> DPGCSELIQASSRITTCSTEGVNTKCRLSGTALIRAGSVGAEACLMLKGVKEDQTKFLKIKTVSSELSCREGQSYWTGSFSPKCLSSRRCHLVGECHVNRCLSW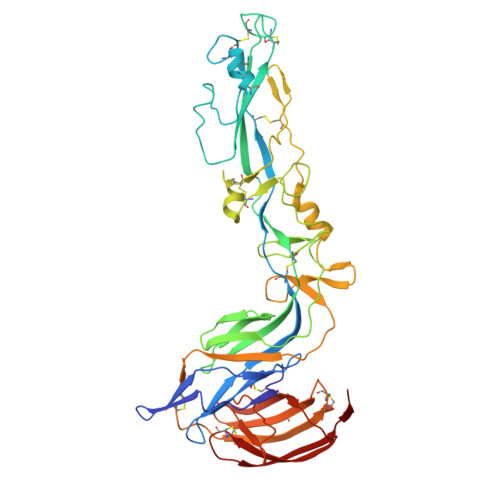RDNETSAEFSFVGESTTMRENKCFEQCGGWGCGCFNVNPSCLFVHTYLQSVRKEALRVFNCIDWVHKLTLEITDFDGSVSTIDLGASSSRFTNWGSVSLSLDAEGISGSNSFSFIESPGKGYAIVDEPFSEIPRQGFLGEIRCNSESSVLSAHESCLRAPNLISYKPMIDQLECTTNLIDPFVVFERGSLPQTRNDKTFAASKGNRGVQAFSKGSVQADLTLMFDNFEVDFVGAAVSCDAAFLNLTGCYSCNAGARVCLSITSTGTGSLSAHNKDGSLHIVLPSENGTKDQCQILHFTVPEVEEEFMYSCDGDERPLLVKGTLIAID In this work, we exhaustively probe the ability of all 36 immobile HJ sequences to form DNA crystals in two different designed systems. Three separate self-assembling DNA crystal systems are described in this report: the “4 × 5” and “4 × 6” designs (collectively referred to as the 4 × N systems), and a third construct with a “scrambled” sequence variant of the 4 × 6 lattices. Self-assembly was mediated by three constituent oligonucleotides: (S1) containing four sequence repeats of either 5 or 6 bases; (S2) composed of 21 bases containing complementary regions to both (S1); and (S3) which forms the second junction crossover. The HJ serves as the fundamental component at the core of each unit, and the ultimate assembly of the full lattice is facilitated by the complementary 2-base sticky ends that tail each duplex.

The 4 × 5 system robustly crystallized with 75% of the junctions, and we obtained crystals in all but 9 of 36 sequences. Of the resulting structures, 18 exhibited P32 symmetry with average cell dimensions a = b = 68.85 Å c = 60.09 Å, with only nine retaining the original P3221 symmetry with average cell edges a = b = 68.17 Å c = 60.60 Å. Although the cell parameters between the two symmetries were virtually indistinguishable, the differences between the periodicity of the lattices is dramatic, with vastly different cavity sizes.

> GAGCAGACCAG;> ACGTCACTCA;> CTCGT;> TCTGAGTGAGGTCTGC> SLLNSRYKLVCYYTNWSWYRPGIGKYSPEDIDPSLCTHIVYGFAVLGNDGLMTAHDTWSDYDNRFYERVVEYKRYGIKVSLALGGWNDSAGDKYSKLVNDPAARAKFVQHAVAFLEKYGFDGLDLDWEYPKCWQVDCSKGPDSDKQGFADLVHELSAVLKPKGLLLSAAVSPNKMVIDAGYDVPVLARLLDWIAVMTYDYHGQWDKKTGHVAPLYYHPDDDTTYFNANYTIHYWMEKGTPASKIVMGMPMYGQSFTIENRGIHGLNIPVSDGGEPGEYTRAKGFLAYYEICDRIRNSGWTVVKDPYQRMGPYAYKGNQWVSFDDVEIIKKKVNFIKSLNLGGGMIWALDLDDYRNRCGQGKHPLLNAIKTELLNPKIE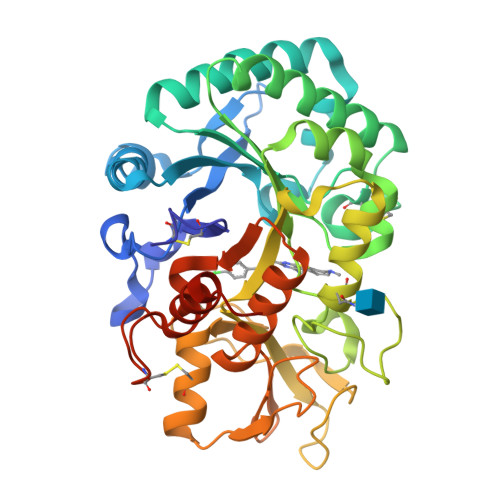MEKEMQQKPHK>[2x]MTDLNIPHTHAHLVDAFQALGIRAGQALMLHASVKAVGAVMGGPNVILQALMDALTPDGTLMMYAGWQDIPDFIDSLPDALKAVYLEQHPPFDPATARAVRENSVLAEFLRTWPCVHRSANPEASMVAVGRQAALLTANHALDYGYGVESPLAKLVAIEGYVLMLGAPLDTITLLHHAEYLAKMRHKNVVRYPCPILRDGRKVWVTVEDYDTGDPH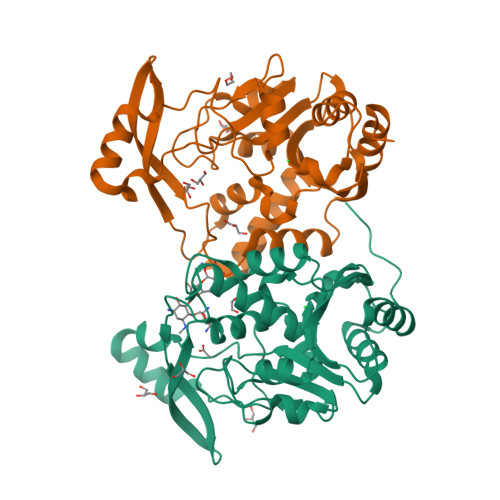DDYSFEQIARDYVAQGGGTRGKVGDADAYLFAAQDLTRFAVQWLESRFGDSAS>SKVVYVSHDGTRRELDVADGVSLMQAAVSNGIYDIVGDCGGSASCATCHVYVNEAFTDKVPAANER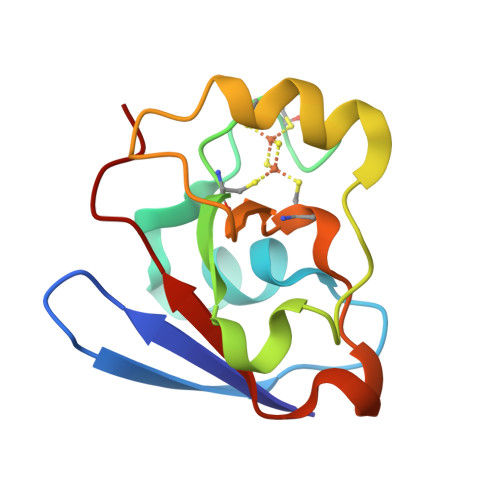EIGMLESVTAELKPNSRLSCQIIMTPELDGIVVDVPDRQW[2x]>[5x]DYKDDDDKLHSQANLM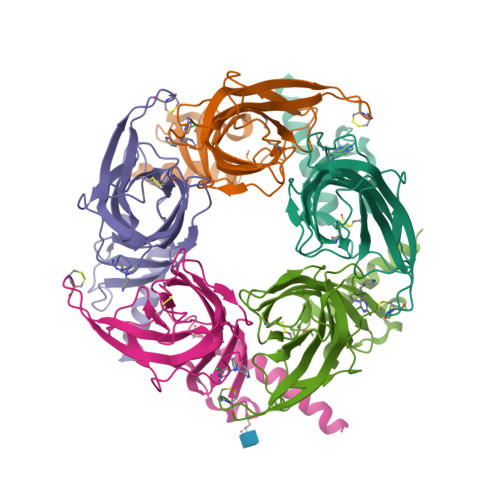RLKSDLFNRSPMYPGPTKDDPLTVTLGFTLQDIVKADSSTNEVDLVYYEQQRWKLNSLMWDPNEYGNITDFRTSAADIWTPDITAYSSTRPVQVLSPQIAVVTHDGSVMFIPAQRLSFMCDPTGVDSEEGATCAVKFGSWVYSGFEIDLKTDTDQVDLSSYYASSKYEILSATQTRQVQHYSCCPEPYIDVNLVVKFRERRAGNGFFRNLFDSR> KDFVRPKLVTIIRSGVKPRKAVRVLLNKKTAHSFEQVLTDITEAIKLETGVVKKL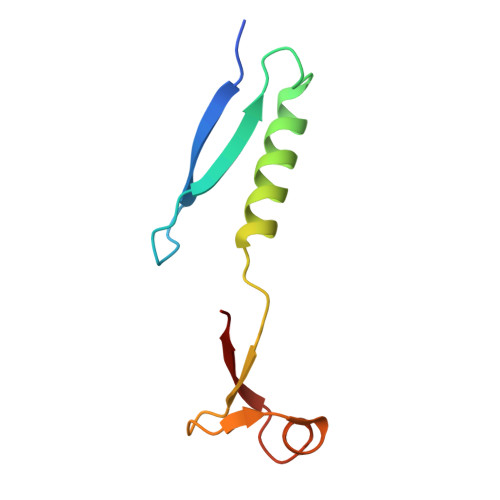YTLDGKQVTCLHDFFGDDDVFIACGP N-[4-(3-chloranyl-4-cyano-phenoxy)-3,5-dimethoxy-phenyl]-1,1,1-tris(fluoranyl)methanesulfonamide 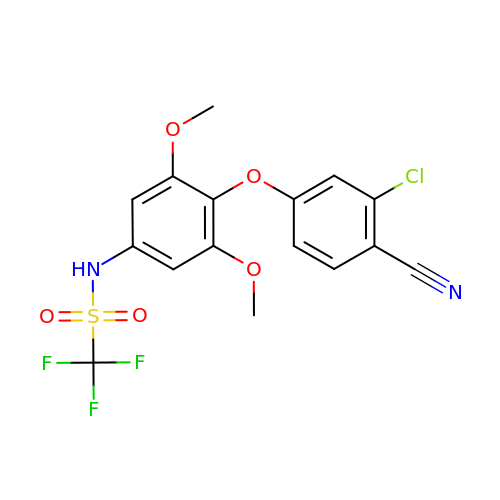| C16 H12 Cl F3 N2 O5 S | LUIIPCXBEHYHFN-UHFFFAOYSA-N> MRGSHHHHHHGSMAERKGTAKVDFLKKIEKEIQQKWDTERVFEVNASNLEKQTSKGKYFVTFPYPYMNGRLHLGHTFSLSKCEFAVGYQRLKGKCCLFPFGLHCTGMPIKACADKLKREIELYGCPPDFPDEEEEEEETSVKTEDIIIKDKAKGKKSKAAAKAGSSKYQWGIMKSLGLSDEEIVKFSEAEHWLDYFPPLAIQDLKRMGLKVDWRRSFITTDVNPYYDSFVRWQFLTLRERNKIKFGKRYTIYSPKDGQPCMDHDRQTGEGVGPQEYTLLKLKVLEPYPSKLSGLKGKNIFLVAATLRPETMFGQTNCWVRPDMKYIGFETVNGDIFICTQKAARNMSYQGFTKDNGVVPVVKELMGEEILGASLSAPLTSYKVIYVLPMLTIKEDKGTGVVTSVPSDSPDDIAALRDLKKKQALRAKYGIRDDMVLPFEPVPVIEIPGFGNLSAVTICDELKIQSQNDREKLAEAKEKIYLKGFYEGIMLVDGFKGQKVQDVKKTIQKKMIDAGDALIYMEPEKQVMSRSSDECVVALCDQWYLDYGEENWKKQTSQCLKNLETFCEETRRNFEATLGWLQEHACSRTYGLGTHLPWDEQWLIESLSDSTIYMAFYTVAHLLQGGNLHGQAESPLGIRPQQMTKEVWDYVFFKEAPFPKTQIAKEKLDQLKQEFEFWYPVDLRVSGKDLVPNHLSYYLYNHVAMWPEQSDKWPTAVRANGHLLLNSEKMSKSTGNFLTLTQAIDKFSADGMRLALADAGDTVEDANFVEAMADAGILRLYTWVEWVKEMVANWDSLRSGPASTFNDRVFAS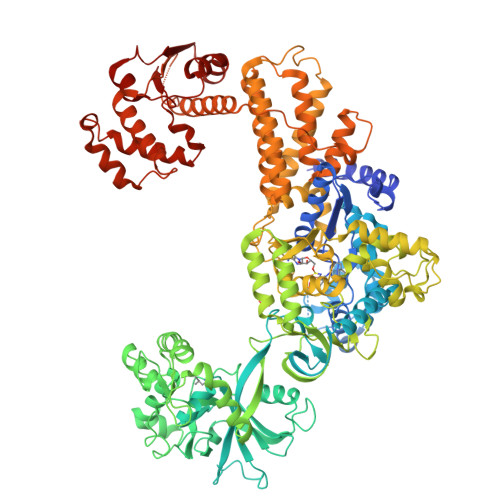ELNAGIIKTDQNYEKMMFKEALKTGFFEFQAAKDKYRELAVEGMHRELVFRFIEVQTLLLAPFCPHLCEHIWTLLGKPDSIMNASWPVAGPVNEVLIHSSQYLMEVTHDLRLRLKNYMMPAKGKKTDKQPLQKPSHCTIYVAKNYPPWQHTTLSVLRKHFEANNGKLPDNKVIASELGSMPELKKYMKKVMPFVAMIKENLEKMGPRILDLQLEFDEKAVLMENIVYLTNSLELEHIEVKFASEAEDKIREDCCPGKPLNVF> GSMPMYEVQWKVVEESNGNNYSYIDPTQLPYDHKWEFPRNRLSFGKTLGAGAFGKVVEATAQGLIKSDAAMTVAVKMLKPSAHSTEREALMSELKVLSYLGNHENIVNLLGACTHGGPTLVITEYCCYGDLLNFLRRKRDEFVPYKVAPEDLYKDFLTLEHLLSFSYQVAKGMAFLASKNCIHRDLAARNILLTHGNITKICDFGLARDIKNDSNYVDKGNARLPVKWMAPESIFNSVYTFESDVWSYGIFLWELFSLGSSPYPGMPVDSKFYKMIKEGFRMSSPEYAPAEMYDIMKTCWDADPDKRPTFKQIVQDIEKQISESTNH

Avapritinib is the only potent and selective inhibitor approved for the treatment of D842V-mutant gastrointestinal stromal tumors (GIST), the most common primary mutation of the platelet-derived growth factor receptor α (PDGFRA). Against this background, we solve the crystal structures of avapritinib in complex with wild-type and mutant PDGFRA and stem cell factor receptor (KIT), which provide evidence and understanding of inhibitor binding and lead to the identification of a sub-pocket (Gα-pocket). Furthermore, we report the identification of a sub-pocket (Gα-pocket) located in the N-lobe of the kinase domain, which is surrounded by amino acids of key regulatory elements such as the Gly-rich loop and the αC-helix.

In general, all derivatives with modifications of the primary amine demonstrated strong inhibitory activities. To our delight, we were able to obtain co-crystal structures at high resolutions for each of the inhibitors 8-12 bound to KIT-wt (1.5–2.0 Å) and 9 bound to PDGFRA-T674I (2.6 Å). While the biochemical evaluation still revealed IC50 values in the sub-nanomolar range, blocking the ability for proton donation through H-bonding by double methylation was accompanied by a slight loss of potency by 3–5-fold. Lower inhibitory activity was observed in KIT cell lines for both alkylated derivatives 8 and 9 compared to PDGFRA cell lines.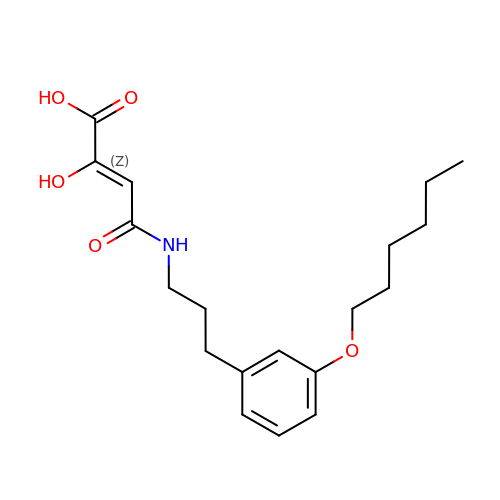(2Z)-4-({3-[3-(hexyloxy)phenyl]propyl}amino)-2-hydroxy-4-oxobut-2-enoic acid | C19 H27 N O5 | LTXZSLKTHFHDTP-VKAVYKQESA-N(1~{R},3~{R})-5-[(2~{E})-2-[(1~{R},3~{a}~{S},7~{a}~{R})-1-[(2~{R},3~{S})-3-[(3~{S})-3-(4-hydroxyphenyl)-3-methoxy-propyl]heptan-2-yl]-7~{a}-methyl-2,3,3~{a},5,6,7-hexahydro-1~{H}-inden-4-ylidene]ethylidene]-2-methylidene-cyclohexane-1,3-diol | C36 H54 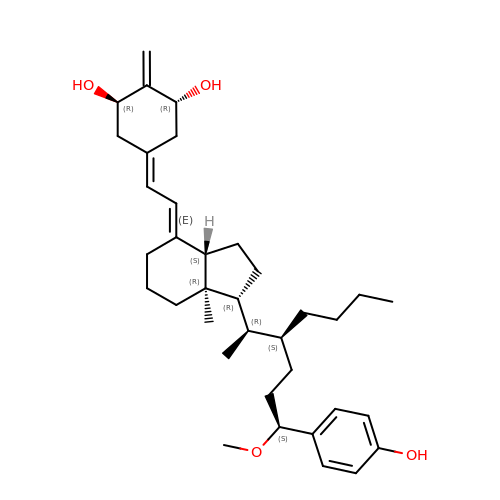O4 | AJZMBYIVQYCFHK-WPVJRCGCSA-N Clostridioides difficile causes life-threatening gastrointestinal infections. Herein, we report 30 X-ray structures from a structure genomics pipeline spanning 13 years, representing 10.2% of the X-ray structures for this important pathogen. The Center for Structural Biology of Infectious Diseases (CSBID, formerly the Center for Structural Genomics of Infectious Diseases) implemented a structural biology pipeline starting in 2010 through paired efforts with systems biology, bioinformatics, and other research specialists in C. difficile pathogenesis. This project ultimately involved 335 proteins linked with pathogenesis, metabolism, and antimicrobial resistance.

The structures presented here are part of the C. difficile 630, R20291, and Y384 sets nominated at CSBID. The overall success of structure determination for C. difficile in both CSBID pipelines was 7%, with a total of 23 unique structures and eight variants or ligand-bound proteins determined.

>MVDYSDCFEGISGGAIFYNTKNKEYNIYNKELIETRRSPASTFKIVSTLIGLEKGVINSKESVMGYDGTEYPNKNWNKNLSLEEAFKESCVWYYKKLIDKVDAKSVQNILDDLKYGNCDISEWEGDLKNGKGHLNGFWLESSLQISPKEQVQTMAKIFEGDTNFKKEHINILRDIMKIDVNDKNINVYGKTGTGFDEKNKRVDAWFVGMLEREGDTYYFAIKSDDSNKEITGPKVKEIAINIIKKYYSVREGAAL[4x]N-(CHLOROPHENYL)-N'-HYDROXYGUANIDINE | C7 H8 Cl N3 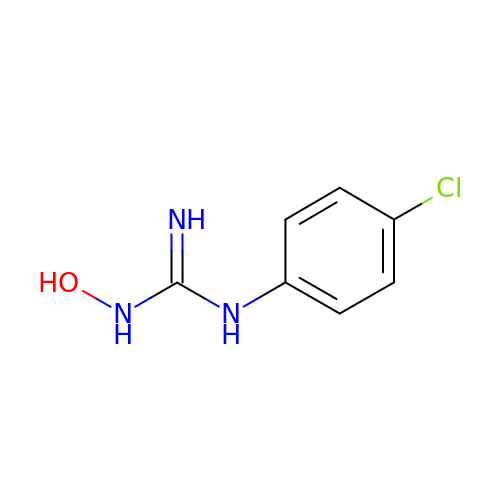O | JYBXKTLYOMPMQY-UHFFFAOYSA-N> MAYPGHPGAG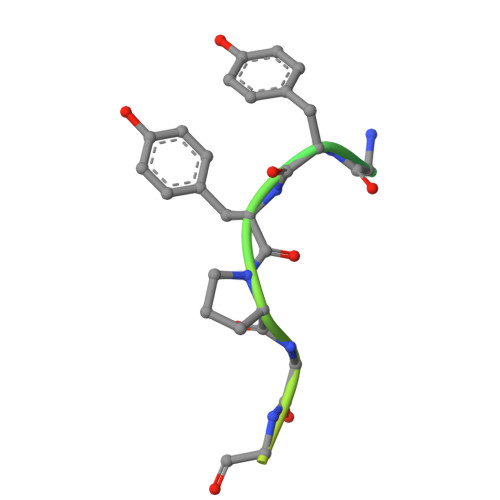GGYYPGGYGGAPGGPAFPGQTQ> GMETYDVLVVGGGPGGSTAARYAAKYGLKTLMIEKRPEIGSPVRCGEGLSKGILNEADIKADRSFIANEVKGARIYGPSEKRPIILQSEKAGNEVGYVLERDKFDKHLAALAAKAGADVWVKSPALGVIKENGKVAGAKIRHNNEIVDVRAKMVIAADGFESEFGRWAGLKSVILARNDIISALQYRMINVDVDPDYTDFYLGSIAPAGYIWVFPKGEGMANVGIGSSINWIHNRFELKNYLDRFIENHPGLKKGQDIQLVTGGVSVSKVKMPITMPGLMLVGDAARLIDPITGGGIANAIVSGMYAAQVTKEAIESNDYSPQMMQKYEKLIKERFERKHLRN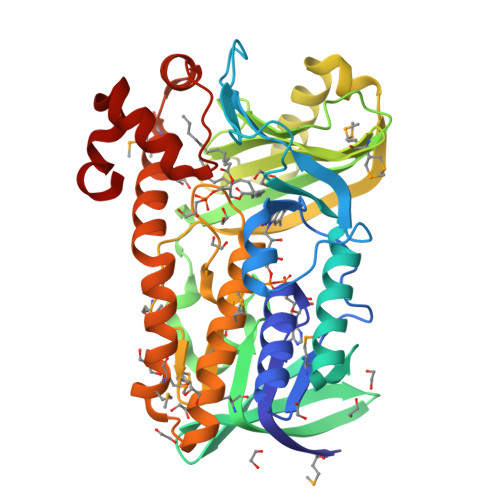WVAKEKLAMLSDDTLDKLVDIVSEQVLTTISVEAILKAIAEKYPEVVKELEDLI>MPRTLAFVSTLLLAAFCALPAQADSFIMRLLNKPVPGGVAVVDLGEEGPPPRAFYQGKPVLVVREEGRRWIAVVGIPLSTKPGPQKLEVRAATGNHEERFSVGSKHYREQRITLKNKRQVNPLPEDLKRIERELAEQTAAYRRFSPGLPSNLMLDKPVDGPLSSPFGLRRFFNGEERNPHSGLDFAVPAGTPIKAPAAGKVILIGD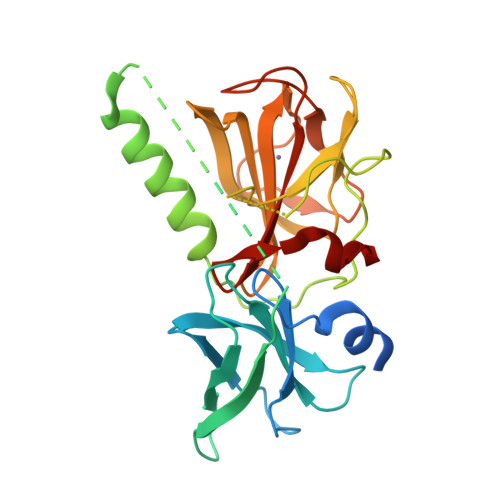YFFNGKTVFVDHGQGFISMFCHLSKIDVKLGQQVPRGGVLGKVGATGRATGPHMHWNVSLNDARVDPAIFIGAFQP[2x]> GIDPFTEFSLESYAFNMKATVEDEKLQGKINDEDKQKILDKCNEIINWLDKNQTAEKEEFEHQQKELEKVCNPIITKLYQSAGGM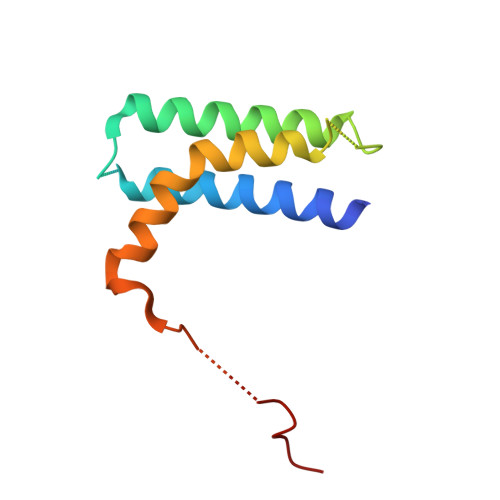PGGMPGGFGPTIEEVD>[4x]SPVENRPLAQKPALTKEALLTGSFFKDVETYTNDQLIGRDELIKNYTIAQINMGKSLINDIILTDDKWLLKNPAWTKKYNEIEQSMPAINDLSQFLKEQNVEFYFALPPSKTNALSFKLPSHIHTYAQENLN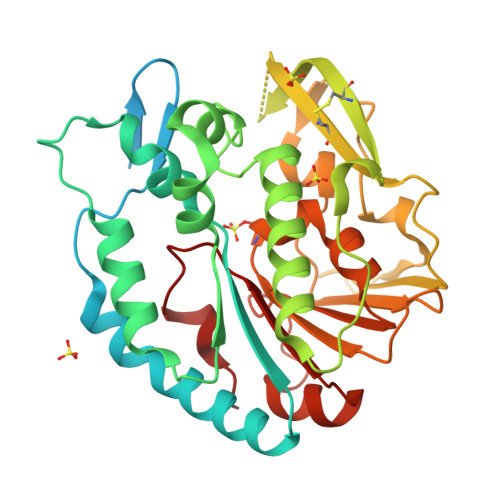YFLKKLPADVKPIKLMEHFKQNYTNEEIQDMYFKTDHHWNMDGAFLGYQYIMNTIGQQSSIYKGKEIAAADYTRTCAQNKHLVGSFNNQLYQLIDANGEKLCYYTPKDGFNFTSVTAKDVQGTVHQNLDEIYGVEAAADTTSYAGYYTDDYPEIVIENNNAQNEVRALVLKDSFANAIVPHLAQSFKHTSILDLRHYHEKDVYQYIQDNNINMVLFVYSDSNLSGDMFKFKK>ASQPNSSAKKKEEKGKNIQVVVRCRPFNLAERKASAHSIVECDPVRKEVSVRTGGLADKSSRKTYTFDMVFGASTKQIDVYRSVVCPILDEVIMGYNCTIFAYGQTGTGKTFTMEGERSPNEEYTWEEDPLAGIIPRTLHQIFEKLTDNGTEFSVKVSLLEIYNEELFDLLNPSSDVSERLQMFDDPRNKRGVIIKGLEEITVHNKDEVYQILEKGAAKRTTAATLMNA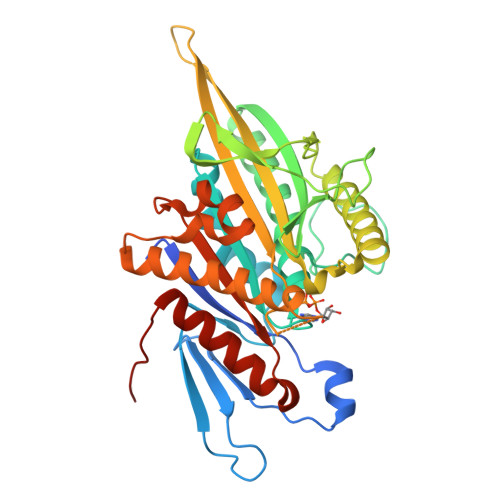YSSRSHSVFSVTIHMKETTIDGEELVKIGKLNLVDLAGSENIGRSGAVDKRAREAGNINQSLLTLGRVITALVERTPHVPYRESKLTRILQDSLGGRTRTSIIATISPASLNLKETLSTLEYAHRAKNILNKPEVNQK[2x]6-HYDROXY-D-NORLEUCINE | C6 H13 N O3 | 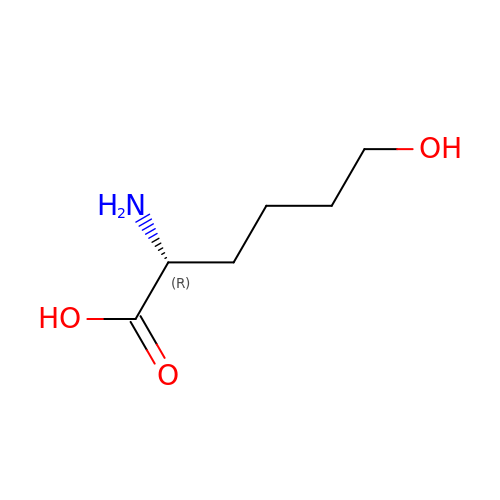OLUWXTFAPJJWPL-RXMQYKEDSA-N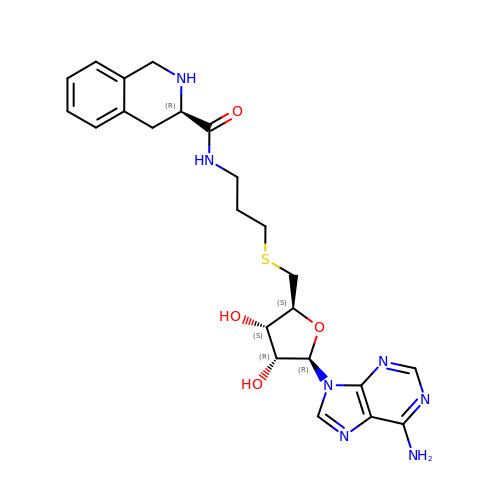5'-S-(3-{[(3R)-1,2,3,4-tetrahydroisoquinolin-3-ylcarbonyl]amino}propyl)-5'-thioadenosine | C23 H29 N7 O4 S | HMZSUDMWDJASBZ-AXKRAVOISA-N>GSFTARPSSSMADFRKFFAKAKHIVIISGAGVSAESGVPTFRGAGGYWRKWQAQDLATPLAFAHNPSRVWEFYHYRREVMGSKEPNAGHRAIAECETRLGKQGRRVVVITQNIDELHRKAGTKNLLEIHGSLFKTRCTSCGVVAENYKSPICPALSGKGAPEPGTQDASIPVE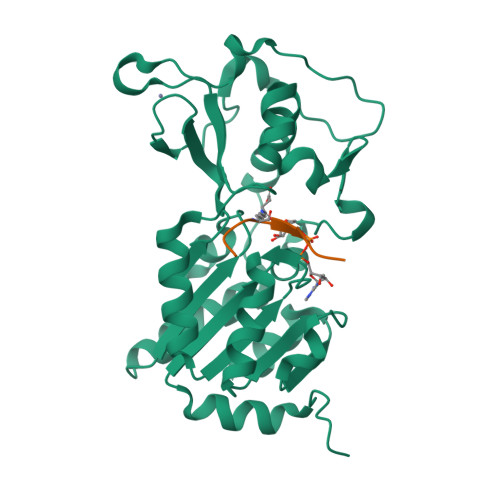KLPRCEEAGCGGLLRPHVVWFGENLDPAILEEVDRELAHCDLCLVVGTSSVVYPAAMFAPQVAARGVPVAEFNTETTPATNRFRFHFQGPCGTTLPEALA[2x];>KQTARXSTGGKA[2x]> MSSATASIKLSNGVEMPVIGLGTWQSSPAEVITAVKTAVKAGYRLIDTASVYQNEEAIGTAIKELLEEGVVKREELFITTKAWTHELAPGKLEGGLRESLKKLQLEYVDLYLAHMPAAFNDDMSEH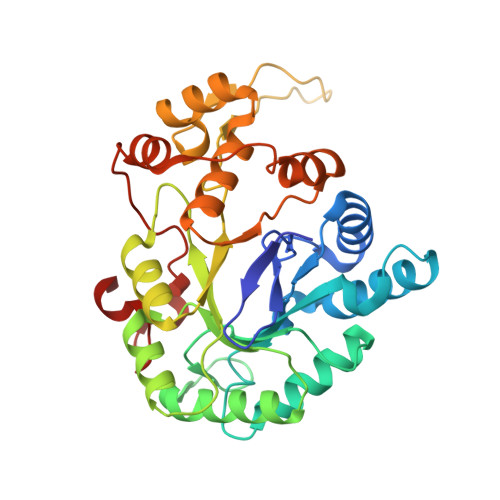IASPVEDVWRQFDAVYKAGLAKAVGVSNWNNDQISRALALGLTPVHNSQVELHLYFPQHDHVDFCKKHNISVTSYATLGSPGRVNFTLPTGQKLDWAPAPSDLQDQNVLALAEKTHKTPAQVLLRYALDRGCAILPKSIQENRIKENFEVFDFSLTEEDIAKLEESKNSQRLFLQDFMTGHPEDAFAAERK> MKSDFKFSNLLGTVYRQGNITFSDDGKQLLSP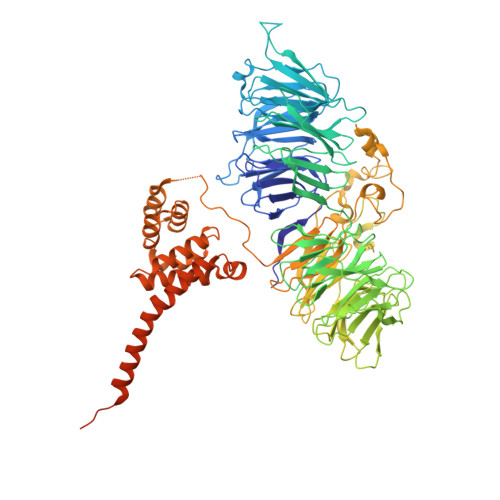VGNRVSVFDLINNKSFTFEYEHRKNIAAIDLNKQGTLLISIDEDGRAILVNFKARNVLHHFNFKEKCSAVKFSPDGRLFALASGRFLQIWKTPDVNKDRQFAPFVRHRVHAGHFQDITSLTWSQDSRFILTTSKDLSAKIWSVDSEEKNLAATTFNGHRDYVMGAFFSHDQEKIYTVSKDGAVFVWEFTKRPSDDDDNESEDDDKQEEVDISKYSWRITKKHFFYANQAKVKCVTFHPATRLLAVGFTSGEFRLYDLPDFTLIQQLSMGQNPVNTVSVNQTGEWLAFGSSKLGQLLVYEWQSESYILKQQGHFDSTNSLAYSPDGSRVVTASEDGKIKVWDITSGFCLATFEEHTSSVTAVQFAKRGQVMFSSSLDGTVRAWDLIRYRNFRTFTGTERIQFNCLAVDPSGEVVCAGSLDNFDIHVWSVQTGQLLDALSGHEGPVSCLSFSQENSVLASASWDKTIRIWSIFGRSQQVEPIEVYSDVLALSMRPDGKEVAVSTLKGQISIFNIEDAKQVGNIDCRKDIISGRFNQDRFTAKNSERSKFFTTIHYSFDGMAIVAGGNNNSICLYDVPNEVLLKRFIVSRNMALNGTLEFLNSKKMTEAGSLDLIDDAGENSDLEDRIDNSLPGSQRGGDLSTRKMRPEVRVTSVQFSPTANAFAAASTEGLLIYSTNDTILFDPFDLDVDVTPHSTVEALREKQFLNALVMAFRLNEEYLINKVYEAIPIKEIPLVASNIPAIYLPRILKFIGDFAIESQHIEFNLIWIKALLSASGGYINEHKYLFSTAMRSIQRFIVRVAKEVVNTTTDNKYTYRFLVSTDGSMEDGAADDDEVLLKDDADEDNEENEENDVVMESDDEEGWIGFNGKDNKLPLSNENDSSDEEENEKELP>MEEPEEPADSGQSLVPVYIYSPEYVSMCDSLAKIPKRASMVHSLIEAYALHKQMRIVKPKVASMEEMATFHTDAYLQHLQKVSQEGDDDHPDSIEYGLGYDCPATEGIFDYAAAIGGATITAAQCLIDGMCKVAINWSGGWHHAKKDEASGFCYLNDAVLGILRLRRKFERILYVDLDLHHGDGVEDAFSFTSKVMTVSLHKFSPGFFPGTGDVSDVGLGKGRYYSVNVPIQDGIQDEKYYQICESVLKEVYQAFNPKAVVLQLGADTIAGDPMCSFNMTPVGIGKCLKYILQWQLATLIL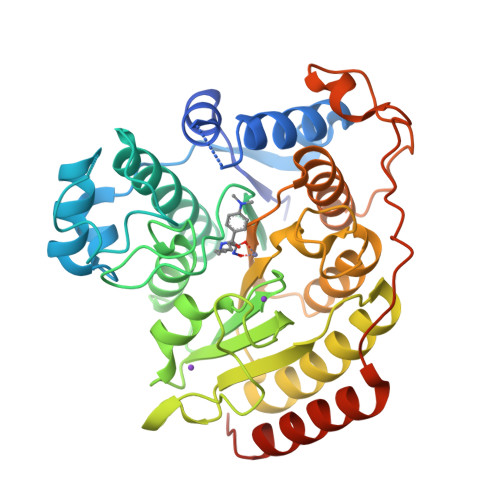GGAGYNLANTARCWTYLTGVILGKTLSSEIPDHEFFTAYGPDYVLEITPSCRPDRNEPHRIQQILNYIKGNLKHVVIEGRGSHHHHHH[2x]>[2x]MAPEINLPGPMSLIDNTKGQLVVNPEALKILSAITQPVVVVAIVGLYRTGKSYLMNKLAGKKNGFSLGSTVKSHTKGIWMWCVPHPKKPEHTLVLLDTEGLGDIEKGDNENDSWIFALAILLSSTFVYNSMGTINQQAMDQLHYVTELTDRIKANSSPGNNSVDDSADFVSFFPAFVWTLRDFTLELEVDGEPITADDYLELSLKLRKGTDKKSKSFNDPRLCIRKFFPKRKCFVFDWPAPKKYLAHLEQLKEEELNPDFIEQVAEFCSYILSHSNVKTLSGGIPVNGPRLESLVLTYVNAISSGDLPCRENAVLALAQIENSAAVEKAIAHYEQQMGQKVQLPTETLQELLDLHRDSEREAIEVFMKNSFKDVDQMFQRKLGAQLEARRDDFCKQNSKASSDCCMALLQDIFGPLEEDVKQGTFSKPGGYRLFTQKLQELKNKYYQVPRKGIQAKEVLKKYLESKEDVADALLQTDQ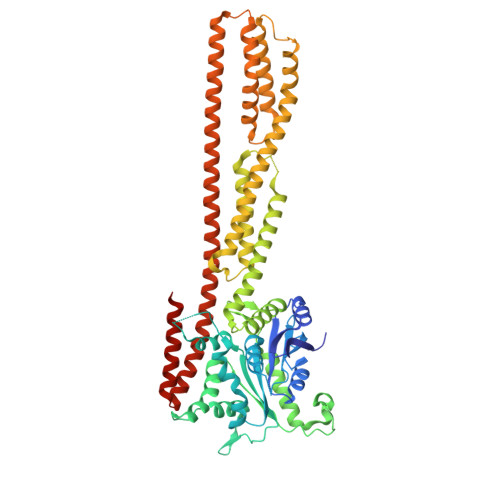SLSEKEKAIEVERIKAESAEAAKKMLEEIQKKNEEMMEQKEKSYQEHVKQLTEKMERDRAQLMAEQEKTLALKLQEQERLLKEGFENESKRLQKDIWDIQMRSKSLEPICNIL PRCP is a lysosomal, serine carboxypeptidase that cleaves hydrophobic C-terminal amino acids adjacent to proline. The S28 family of peptidases consists of two enzymes, PRCP and DPP7. PRCP contains an α/β hydrolase domain harboring the catalytic Asp-His-Ser triad and a novel helical structural domain that caps the active site. PRCP was originally discovered as an angiotensinase and has since been implicated in vasodilatory, proinflammatory, and metabolic pathways.

The crystal structure of human PRCP was determined using MIRAS phasing techniques at 2.8 Å resolution by analyzing native, mercury and platinum-derivatized crystals. Interpretation of heavy-atom positions and resultant electron-density maps show that the asymmetric unit contains one molecule of PRCP with an unusually high solvent content of 82%. The final refined model consists of residues 46-348 and 353-491, five N-linked glycans, and four disulfide bridges (residues 215-372, 233-310, 264-343 and 364-394). Clear evidence of covalently attached and ordered saccharide is observed at the other five canonical glycosylation sites. The overall architecture of PRCP consists of two main structural entities: an α/β hydrolase domain and a novel SKS domain. The first part of the insertion (residues 194-334) consists of five helices packed into a novel helical bundle (the SKS domain) that caps the active site. The catalytic triad consisting of Ser 179, Asp 430 and His 455 can be identified based on structural similarity with other hydrolases. An unanticipated feature of the PRCP active site is an apparent charge-relay system that links the catalytic histidine (His 455) with His 456 and Arg 460. Structural alignments strongly suggest that the hydrophobic pocket in PRCP, formed by Trp 432, Trp 459, Met 183 and Met 369 is functionally equivalent to the S1 binding sites of PEP and DPP4. The binding of known substrates by PRCP that are cleaved at the C-terminus requires access to the long substrate binding groove of PRCP.

> KNYSVLYFQQKVDHFGFNTVKTFNQRYLVADKYWKKNGGSILFYTGNEGDIIWFCNNTGFMWDVAEELKAMLVFAEHRYYGESLPFGDNSFKDSRHLNFLTSEQALADFAELIKHLKRTIPGAENQPVIAIGGSYGGMLAAWFRMKYPHMVVGALAASAPIWQFEDLVPCGVFMKIVTTDFRKSGPHCSESIHRSWDAINRLSNTGSGLQWLTGALHLCSPLTSQDIQHLKDWISETWVNLAMVDYPYASNFLQPLPAWPIKVVCQYLKNPNVSDSLLLQNIFQALNVYYNYSGQVKCLNISETATSSLGTLGWSYQACTEVVMPFCTNGVDDMFEPHSWNLKELSDDCFQQWGVRPRPSWITTMYGGKNISSHTNIVFSNGELDPWSGGGVTKDITDTLVAVTISEGAHHLDLRTKNALDPMSVLLARSLEVRHMKNWIRDFYDS>[4x]MGHHHHHHMTDLEKPNLAGHMFDVVVIGGGISGLAAAKLLSEYKINVLVLEARDRVGGRTYTVRNEHVKWVDVGGAYVGPTQNRILRLSKELGIETYKVNVNERLVQYVKGKTYPFRGAFPPVWNPLAYLDYNNLWRTMDEMGKEIPVDAPWQARHAQEWDKMTMKDLIDKICWT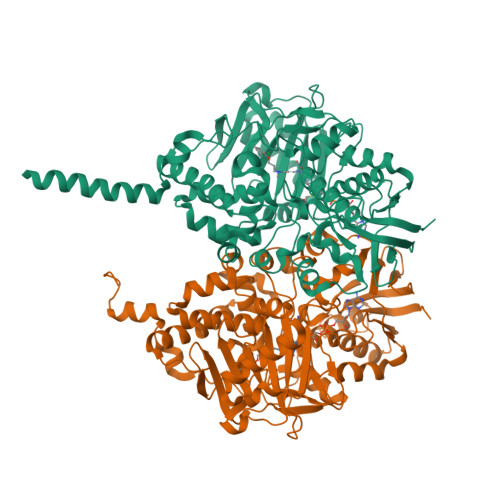KTAREFAYLFVNINVTSEPHEVSALWFLWYVRQCGGTARIFSVTNGGQERKFVGGSGQVSEQIMGLLGDKVKLSSPVTYIDQTDDNIIVETLNHEHYECKYVISAIPPILTAKIHFKPELPPERNQLIQRLPMGAVIKCMVYYKEAFWKKKDYCGCMIIEDEEAPIAITLDDTKPDGSLPAIMGFILARKADRLAKLHKDIRKRKICELYAKVLGSQEALYPVHYEEKNWCEEQYSGGCYTAYFPPGIMTQYGRVIRQPVGRIYFAGTETATQWSGYMEGAVEAGERAAREVLNALGKVAKKDIWVEEPESKDVPAIEITHTFLERNLPSVPGLLKITGVSTSVALLCFVLYKIKKLPC6-[HYDROXYIMINO-(5,5,8,8-TETRAMETHYL-5,6,7,8-TETRAHYDRO-NAPHTALEN-2-YL)-METHYL]-NAPHTALENE-2-CARBOXYLIC 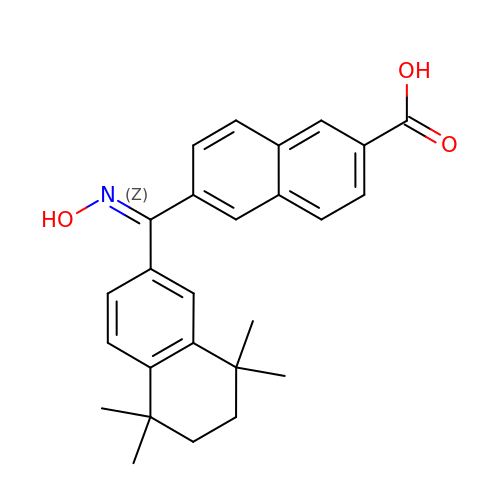ACID | C26 H27 N O3 | RNZIUDLOJHVHLZ-SLEBQGDGSA-N> MERPQLDSMSQDLSEALKEATKEVHIRAENSEFMRNFQKGQVSREGFKLVMASLYHIYTALEEEIERNKQNPVYAPLYFPEELHRRAALEQDMAFWYGPHWQEAIPYTPATQHYVKRLHEVGGTHPELLVAHAYTRYLGDLSGGQVLKKIAQKAMA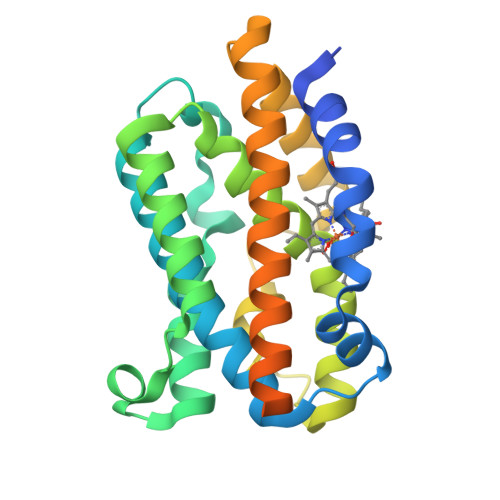LPSSGEGLAFFTFPSIDNPTKFKQLYRARMNTLEMTPEVKHRVTEEAKTAFLLNIELFEELQALLTEEHKDQSPSQTEFLRQRPASLVQDTTSAETPRGKSQISTSSSQTP> GPGGEMQKIVFKI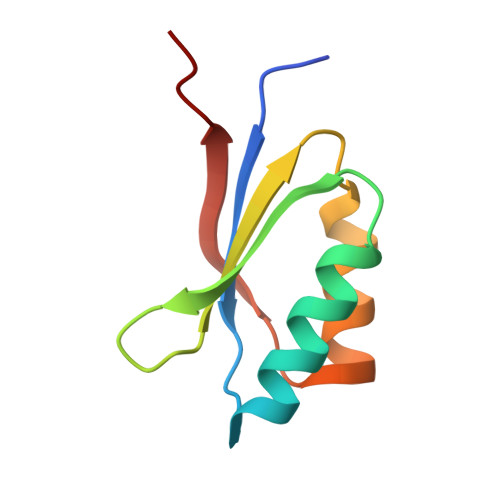PMVDDKSRTKAMSLVASTVGVHSVAIAGDLRDQVVVVGDGIDSINLVSALRKKVGPAMFLEVSQVKED> MQSTLVIAEHANDSLAPITLNTITAATRLGGEVSCLVAGTKCDKVAQDLCKVAGIAKVLVAQHDVYKGLLPEELTPLILATQKQFNYTHICAGASAFGKNLLPRVAAKLEVAPISDIIAIKSPDTFVRTIYAGNALCTVKCDEKVKVFSVRGTSFDAAATSGGSASSEKASSTSPVEISEWLDQKLTKSDRPELTGAKVVVSGGRGLKSG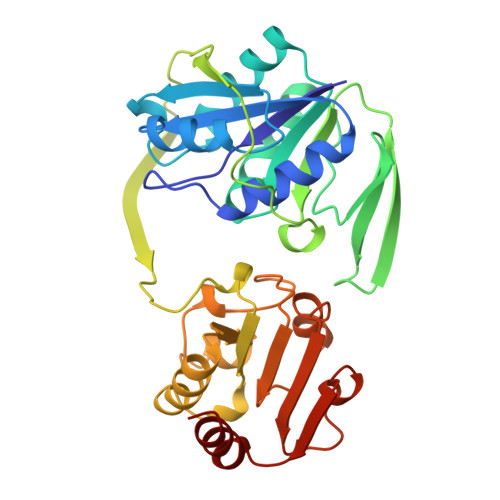ENFKLLYDLADQLHAAVGASRAAVDAGFVPNDMQVGQTGKIVAPELYIAVGISGAIQHLAGMKDSKTIVAINKDPEAPIFQVADYGIVADLFKVVPEMTEILKKK>[2x]SNAMILDKIFEKTKEDLKERKLKLPYDMLGRSLASNPFFPKDVIKALKRVEKEVKIIAEVKKASPSKGVIREDFDPLSIALNYEKNKAAAISVLTEPHFFKGSLEYLSLIRRYTQIPLLRKDFIFDEYQILEALVYGADFVLLIAKMLSMKELKKLLEFARHLGLEALVEIHDKEDLSKAIFAGADIIGINHRNLEDFTMDMSLCEKLIPQIPNSKIIIAESGLENKEFLEHLQNLGVDAFL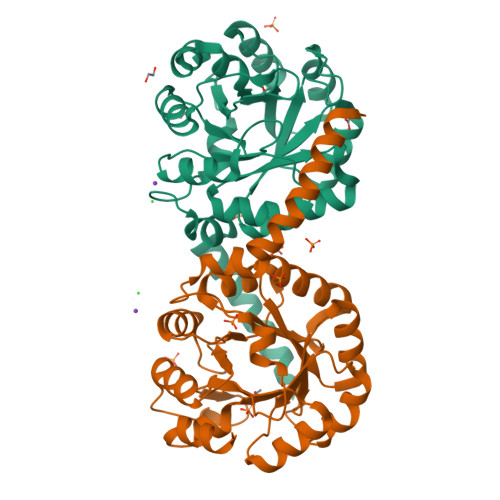IGEYFMREKDEGKALKALL> DKAMAGNFWQSSHYLQWILDKQDLLKERQKDLKFLSEEEYWKLQIFFTNVIQALGEHLKLRQQVIATATVYFKRFYARYSLKSIDPVLMAPTCVFLASKVEEFGVVSNTRLIAAATSVLKTRFSYAFPKEFPYRMNHILECEFYLLELMDCCLIVYHPYRPLLQYVQDMGQEDMLLPLAWRIVNDTYR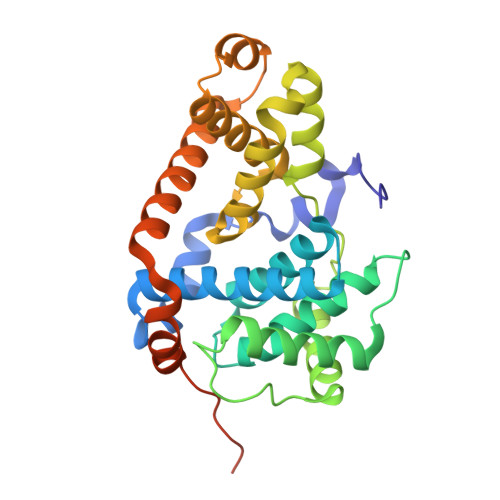TDLCLLYPPFMIALACLHVACVVQQKDARQWFAELSVDMEKILEIIRVILKLYEQWKNFDERKEMATILSKMPKPKPPPNSEGEQGPNGSQNSSYSQS> HTLVWGVWVNGVDQGDGRNIYIRSPPNNNPVKNLTSPDMTCNVDNRVVPKS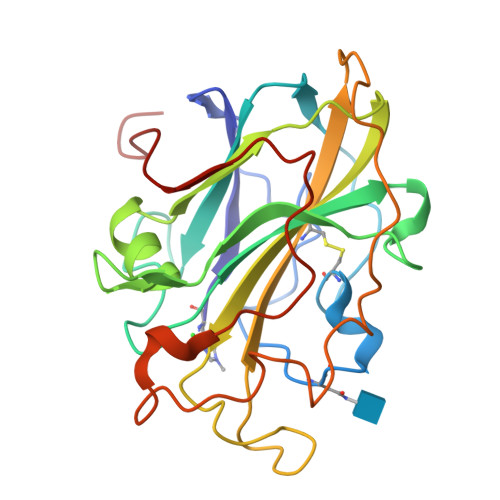VPVNAGDTLTFEWYHNTRDDDIIASSHHGPIAVYIAPAASNGQGNVWVKLFEDAYNVTNSTWAVDRLITAHGQHSVVVPHVAPGDYLFRAEIIALHEADSLYSQNPIRGAQFYISCAQITINSSDDSTPLPAGVPFPGAYTDSTPGIQFNIYTTPATSYVAPPPSVWSGALGGSIAQVGDASLE> PLTNDERQLMHELAVQVVCSQTGCSPDAAVEALESFAKDGTLILRGDTENAYLEAGGNVLVH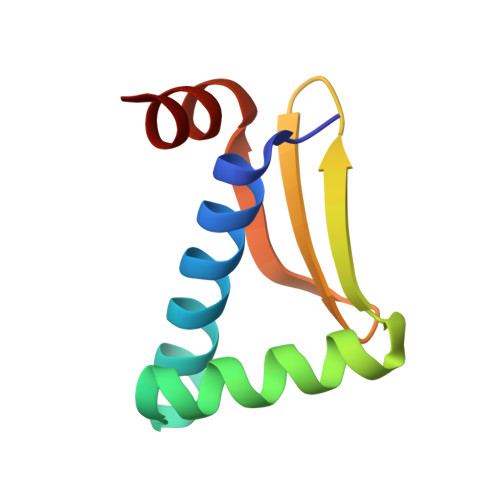ADRDWLAFHASY> MAHHHHHHSSGLEVLFQGPMDAPMEDAPAPVAQVKVIFTTTEPDLELPESKRQLLVPADIRRYGLSRILNSESMLDTGSIPFDFLINGSFLRSSLEDYLTSNGLSLETTLTLQYVRSLIPPVYEASFEHDDWVSAVDVLSATSPAGRWSSAANSSAAVQPGQERVLSASYDGLLRIWNASGSVIATSPSGSHGGHTASIKAAKFLTSDRLASAGMDRTVRVWKYTESDHFTGELKPTLELYGHTGSVDWLDVDGHSKHILTASADGAIGFWSASKASAPEPDASLLPGAHVSKRRKATSSVSTAQRGPLGLWSIHTAPATAAIFDPRDRTVAYSASQDHTVRTLDLTTGQVVSTLTLTHPLLSLSALTRAGTTSPLLAAGTSARHITMVDPRASSATTSVMTLRGHANKVVSLSPSPEN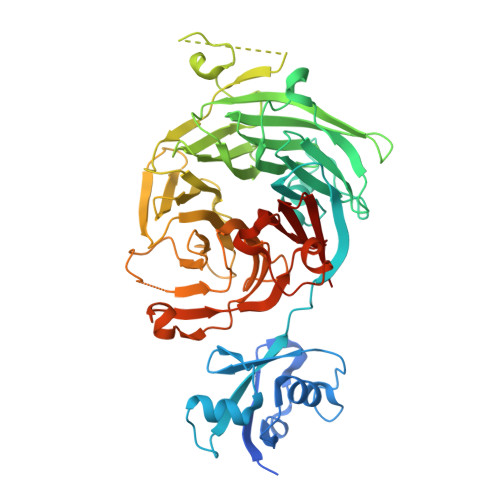EYSLVSGSHDGTCRVWDLRSVRPATKEEGSLGGVSEPVYVIERESWASKGKKKRPVAGDGCKVFSVVWDKLGIFSGGEDKKVQVNRGRNIVTEQK> MGSDKIHHHHHHENL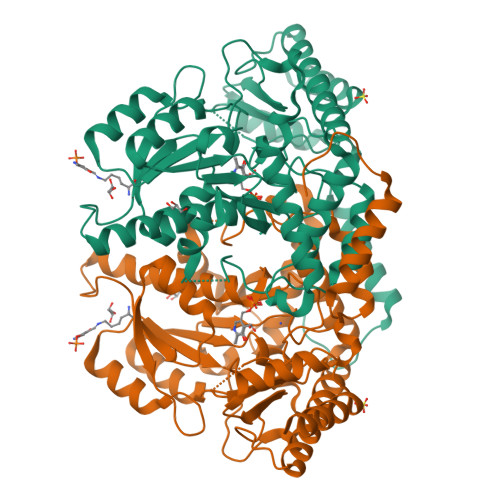YFQGMRNMQEKGVSEKEILEELKKYRSLDLKYEDGNIFGSMCSNVLPITRKIVDIFLETNLGDPGLFKGTKLLEEKAVALLGSLLNNKDAYGHIVSGGTEANLMALRCIKNIWREKRRKGLSKNEHPKIIVPITAHFSFEKGREMMDLEYIYAPIKEDYTIDEKFVKDAVEDYDVDGIIGIAGTTELGTIDNIEELSKIAKENNIYIHVDAAFGGLVIPFLDDKYKKKGVNYKFDFSLGVDSITIDPHAMGHCPIPSGGILFKDIGYKRYLDVDAPYLTETRQATILGTRVGFGGACTYAVLRYLGREGQRKIVNECMENTLYLYKKLKENNFKPVIEPILNIVAIEDEDYKEVCKKLRDRGIYVSVCNCVKALRIVVMPHIKREHIDNFIEILNSIKRD> VAHFTFQPDPEPREYGQTQKMNLFQSVTSALDNSLAKDPTAVIFGEDVAFGGVFRCTVGLRDKYGKDRVFNTPLCEQGIVGFGIGIAVTGATAIAEIQFADYIFPAFDQIV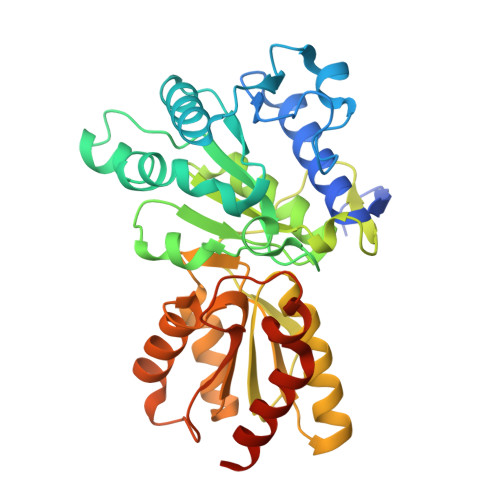NEAAKYRYRSGDLFNCGSLTIRSPWGCVGHGALYHSQSPEAFFAHCPGIKVVIPRSPFQAKGLLLSCIEDKNPCIFFEPKILYRAAAEEVPIEPYNIPLSQAEVIQEGSDVTLVAWGTQVHVIREVASMAKEKLGVSCEVIDLRTIIPWDVDTICKSVIKTGRLLISHEAPLTGGFASEISSTVQEECFLNLEAPISRVCGYDTPFPHIFEPFYIPDKWKCYDALRKMINYGGHHHHHH>QQEATEVRPEQKMPTLLRVYIDGPHGMGKTTTTQLLVALGSRDDIVYVPEPMTYWRVLGASETIANIYTTQHRLDQGEISAGDAAVVMTSAQITMGMPYAVTDAVLAPHIGGEAGSSHAPPPALTLIFDRHPIAALLCYPAARYLMGSMTPQAVLAFVALIPPTLPGTNIVLGALPEDRHIDRLAKRQRPGERLDLAMLAAIRRVYGLLANTVRYLQCGGSWREDWGQLSGTAVPPQGAEPQSNAGPR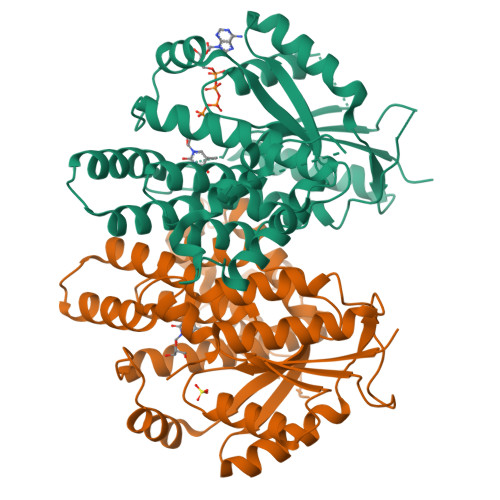PHIGDTLFTLFRAPELLAPNGDLYNVFAWALDVLAKRLRSMHVFILDYDQSPAGCRDALLQLTSGMVQTHVTTPGSIPTICDLARTFAREMGEAN[2x]>MAERPLDVIHRSLDKDVLVILKKGFEFRGRLIGYDIHLNVVLADAEMIQDGEVVKRYGKIVIRGDNVLA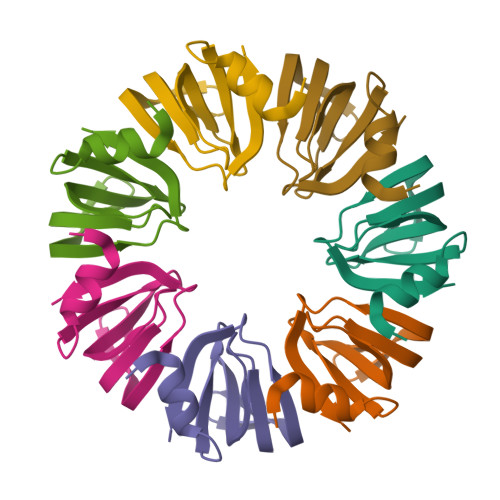ISPTEE[28x]>HMSQSNRELVVDFLSYKLSQKGYSWSQMAAVKQALREAGDEFELRYRRAFSDLTSQLHITPGTAYQSFEQVVNELFRDGVNWGRIVAFFSFGGALCVESVDKEMQVLVSRIAAWMATYLNDHLEPWIQENGGWDTFVELYGNNAAAESRKGQE[2x];>DEMFSDIYKIREIADGLCLEV[6x]

Translationally Controlled Tumor Protein (TCTP/tpt1) is a regulator of pluripotency, the cancer stem cell compartment5, the tumor reversion program, tumor progression and certain forms of inflammatory diseases. TCTP is a major anti-apoptotic protein that exerts its activity on one side by direct binding to Bcl2 family members Mcl1 and Bcl-xL111213 and on the other side by engaging into a reciprocal negative feedback loop with p535. Altogether our results demonstrate that TCTP contains a non-canonical but functional BH3-domain that binds to -and unexpectedly activates- the anti-apoptotic function of Bcl-xL. By using extensive biochemical and biophysical studies we show that TCTP forms heterotetrameric complexes with Bcl-xL via crucial interactions between the N-Terminal region of TCTP (TCTP11–31) and the BH3 binding groove of Bcl-xL.

To provide structural details of the TCTP/Bcl-xL interaction, the crystal structure of a deletion variant of Bcl-xL (Bcl-xLΔ27–81ΔTM) in complex with TCTP11–31 has been solved and refined at 2.1 Å. This crystal structure revealed that upon binding to Bcl-xL, the residues 16–27 of TCTP11–31 completely refold into a 3 turn α-helix conformation that binds to the BH3-binding pocket of Bcl-xL, a hydrophobic groove created by helices α2-α5 of Bcl-xL. In unbound TCTP17, this N-terminal region stabilizes the β-sheet hydrophobic core of the entire TCTP protein. This suggests that the interaction between the full size Bcl-xL and TCTP proteins induces a substantial reorganization of the known TCTP fold. The main difference in the binding of TCTP to the Bcl-xL groove as compared to other high affinity BH3 proteins such as Bax is the absence of the first turn of the helix, located just before the canonical h1 (P1) motif which is non-conserved in TCTP. The side chain of the hydrophobic residues at the h2 (P2, I20), h3 (P3, I23) and h4 (P4, L27) positions form a network of van der Waals interactions with the Bcl-xL groove. Three additional residues, I17, L29 and the side chain of K19 participate in this hydrophobic packing. Of note, since the canonical h1 (P1) is missing in TCTP, I17 might counterbalance this absence by packing with the hydrophobic residues F97, Y101, F105, L108, V126, V141, F146 and Y195 of Bcl-xL in the target-binding pocket formed by helices α2-α5. Furthermore several hydrogen bonds and two salt bridge interactions contribute to the recognition process: (i) R21 of TCTP BH3 domain interacts with E129 and D133 in Bcl-xL; and (ii) D25, part of the (Gly/Ala)-Asp motif between the h3 (P3) and h4 (P4) positions of BH3 domain, interacts with R139 in Bcl-xL.> MVHYKLTYFDGRGAAEIIRQIFVLAGQEYEDIRLSHDEWPKYKNEMPFGQLPVLEVDGKKL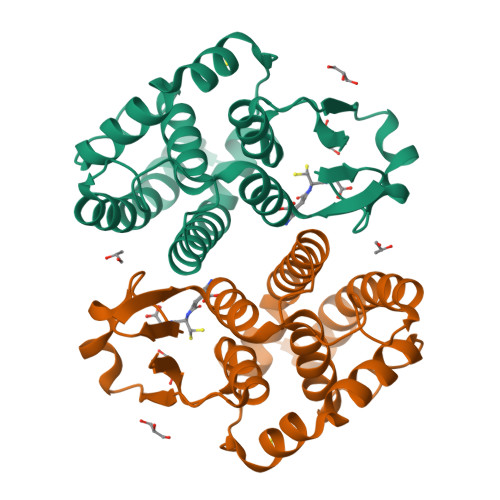AQSFAIARFVAKKFGFAGKCPFEEALVDSITDQYKDFINEIRPFLRVAMGFAEGDLEKLSNEVFLPAREKFFGFMTNFLKESKSGYLVGDSLTFADLYLAECASEFAKKTPTIFDGFPEIKAHAEKVRSNPALKKWIETRPETKF> MVSRYVPDMGDLIWVDFDPTKGSAQAGHRPAVVLSPFMYNNKTGMCLCVPC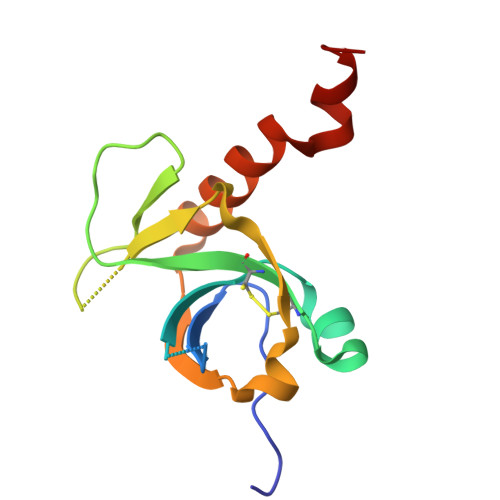TTQSKGYPFEVVLSGQERDGVALADQVKSIAWRARGATKKGTVAPEELQLIKAKINVLIGLSHHHHHH X-ray crystal structures of SamR0483 alone and in complex with hexanoyl-CoA reveal the molecular basis for medium chain acyl-CoA recognition by this unusual YCC β-subunit, prompting us to rename it medium chain acyl-CoA carboxylase beta subunit (MccB). Similar to other bacterial YCC β-subunits, MccB has 3–2 symmetry and is composed of three individual dimers that form a ring-like hexamer. Each monomer can be divided into two domains harbouring two copies of the crotonase fold that pack together in an antiparallel manner to form a dimer. Taken together, these results establish the existence of a unique YCC-dependent pathway for unusual polyketide extender unit biosynthesis.

Given the high degree of structural and sequence similarity between MccB and PccB, it was not immediately clear how the former is able to accommodate significantly longer acyl-CoA substrates than the latter. To address this question structures of MccB bound to either one or four molecules of hexanoyl-CoA were solved to 2.75 and 2.85 Å, respectively. These co-crystal structures were obtained via incubation of MccB with 5 or 10 mM hexanoyl-CoA before crystallization. The hexanoyl-CoA bound structures reveal that some of the substrate-binding features of MccB are similar to those employed by other YCC β-subunits. The residues that interact with hexanoyl-CoA are localized in three regions at the MccB dimer interface. The first region is located at the entrance of the substrate binding pocket, which is characterized by a network of hydrogen bonds between the adenosine moiety of hexanoyl-CoA and the protein. The exocyclic amine and N-1 of adenine form hydrogen bond contacts with the peptide backbone of Ile147, Ala145 and Gly143 monomer B. The second region is the PPant binding site, in which the backbone N-H groups of Ala145 and Gly184 in monomer B form hydrogen bonds to the carbonyl oxygen atom of the β-alanine component of PPant. In addition, the sulfur atom of the thioester is hydrogen bonded to the backbone N-H of Gly420. The third region is the binding pocket for the aliphatic portion of the substrate, which is formed primarily by the hydrophobic side chains of Ile396, Phe399 and Ala423 in Monomer F, and Leu191, Tyr157 and Tyr187 in monomer B.

>[6x]GIDPFTMSLQEPVSPVEESPTSTADRIADLAARHEEAVVLAEKKAADRQHLKGKLTARARIDLLLDPGSFVELDEFVRHRTVEAGIPRPYGDGVVTGHGTIDGRQVCVFSHDFTTLGGSMGEAFGSKVVKIYDFAMSVGCPVIGINDSGGARIQEGVMSIAYYTELGVRNVHSSGVIPQISLIMGPCAGGSVYSPALTDFTVMVKDISYMFVTGPEVVSAVMGEQVTAEQLGGPAVHAEVSGNAHYVGDDEQDAISWVQTLLGYLPPNNLDPAPVYDHDCAPGITEADLALDTVIPDSEQQVYDMADVITAVLDDGDYLEIHPDFARNIICALGRVEGHSVAVVANQPRHLAGVLDIDASEKAARFIRFCDSFNIPVLTFMDVPGYLPGVGQEHQGIIRRGIKLFYAYAESTVPKITVITRKAYGGGYAVMGSRQIGADRVMAWPTAEIAVMGANSAVPILHRRELAAVPPEERAAVKENLVDDYRRRFGNPYEAAAHGYVDMVISPSRTRYEVARALASLRNKRQARPARKHGNIPL>[2x]MNAIGNFLVGTPVFTIFIALALGYLLGKLKIGSFTLGATVGVLIVALLIGQLGVFPRDTCLGDIFFDFFMFAIGYRVGPSFISSMKKFGAKIVYATLIFLVSAFIVAYAAFKMFHIGPGIAAGIIAGGLTQSAVIGSSLETISKLPISDHLKTLYSNQIPIVYTLTYVFGTIGVLIFLRDIMPKLMHIDLKKQAVKTAKELDMIPVPVIVASTHFYTINDGSSLIGQTLGTVNTKFAKGLVAAGLNDSADMASVINAGDVLAISGGIDEIGRAVQEFNLLEVTGKTKAYVSKQVVLKKNFSADVLKNAQDKGVLVATLAGDVMDPAQFSTLHHHHHHKPAESVTLVGQKDAVSEVQSQLGRLRAAENIINYSWFALGIALSAALGIVGTKVSGVPIALGGGTASLIVGLVQSIYRDKHAHMDTIPDSLLEFFQSIGLNLFIATVGLSAAKTFISAIQSMGISVLLIGAVISILPHIITFV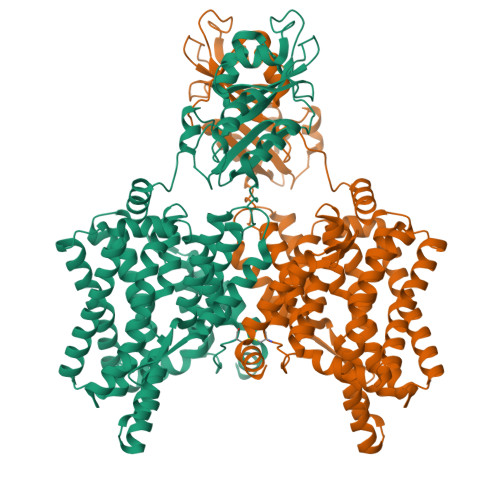IAYYLMKMEPISIIGAQTGADTLSAALNDVSERVGSDASPFFAAAVAPAYAIGNIFLTLMGPIFIVLLS> MTLSPYLQEVAKRRTFAIISHPDAGKTTITEKVLLFGQAIQTAGTVKGRGSNQHAKSDWMEMEKQRGISITTSVMQFPYHDCLVNLLDTPGHEDFSEDTYRTLTAVDCCLMVIDAAKGVEDRTRKLMEVTRLRDTPILTFMNKLDRDIRDPMELLDEVENELKIGCAPITWPIGCGKLFKGVYHLYKDETYLYQSGKGHTIQEVRIVKGLNNPDLDAAVGEDLAQQLRDELELVKGASNEFDKELFLAGEITPVFFGTALGNFGVDHMLDGLVEWAPAPMPRQTDTRTVEASEDKFTGFVFKIQANMDPKHRDRVAFMRVVSGKYEKGMKLRQVRTAKDVVISDALTFMAGDRSHVEEAYPGDILGLHNHGTIQIGDTFTQGEMMKFTGIPNFAPELFRRIRLKDPLKQKQLLKGLVQLSEEGAVQVFRPISNNDLIVGAVGVLQFDVVVARLKSEYNVEAVYESVNVATARWVECADAKKFEEFKRKNESQLALDGGDNLAYIATSMVN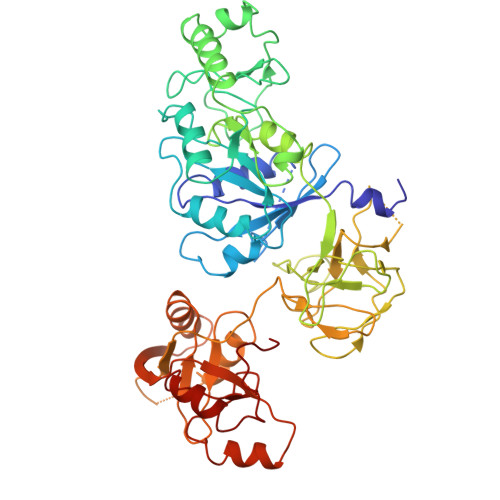LRLAQERYPDVQFHQTREH>[4x]MPVAGSELPRRPLPPAAQERDAEPRPPHGELQYLGQIQHILRCGVRKDDRTGTGTLSVFGMQARYSLRDEFPLLTTKRVFWKGVLEELLWFIKGSTNAKELSSKGVKIWDANGSRDFLDSLGFSTREEGDLGPVYGFQWRHFGAEYRDMESDYSGQGVDQ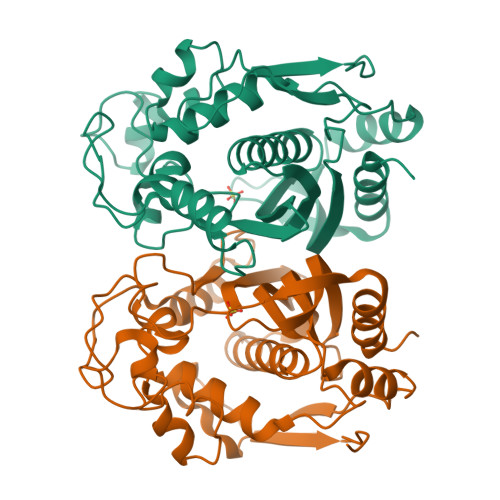LQRVIDTIKTNPDDRRIIMCAWNPRDLPLMALPPCHALCQFYVVNSELSCQLYQRSGDMGLGVPFNIASYALLTYMIAHITGLKPGDFIHTLGDAHIYLNHIEPLKIQLQREPRPFPKLRILRKVEKIDDFKAEDFQIEGYNPHPTIKMEMAVHHHHH>[2x]MSSMTQNLREVMKVMFKVPGFDRVLEKVTLVSAAPEKLICEMKVEEQHTNKLGTLHGGLTATLVDSISTMALMCTERGAPG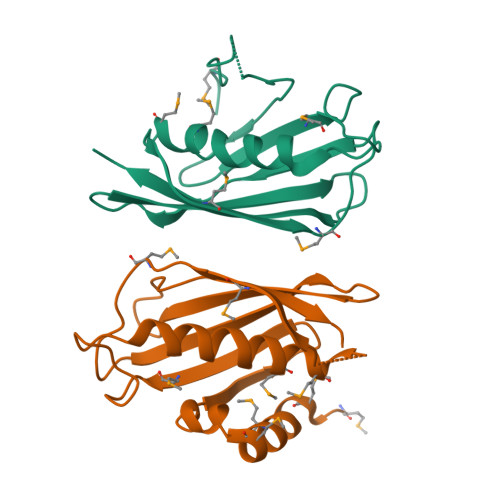VSVDMNITYMSPAKIGEEIVITAHILKQGKTLAFASVDLTNKTTGKLIAQGRHTKHLGN>MVAQQTRTDFDLAQYLQVKKGVVEAALDSSLAIARPEKIYEAMRYSLLAGGKRLRPILCITACELCGGDEALALPTACALEMIHTMSLIHDDLPSMDNDDFRRGKPTNHKVYGEDIAILAGDGLLAYAFEYVVTHTPQADPQALLQVIARLGRTVGAAGLVGGQVLDLESEGRTDITPETLTFIHTHKTGALLEASVLTGAILAGATGEQQQRLARYAQNIGLAFQVVDDILDITATQEELGKTAGKDVKAQKATYPSLLGLEASRAQA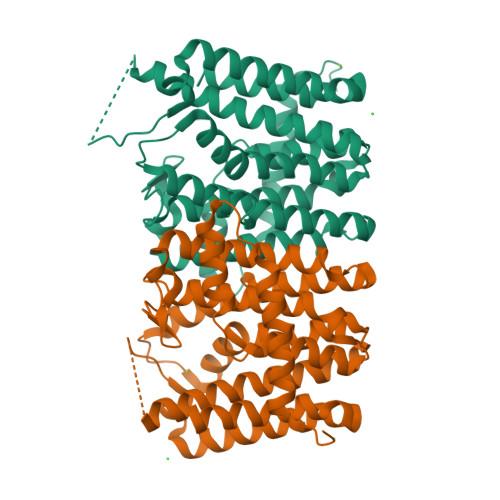QSLIDQAIVALEPFGPSAEPLQAIAEYIVARKYLEHHHHHH[2x]>MDVDLGKLFFCGFDDFNEEAREVIQKYRPAGVLIYPGVLSKEYLFLDFMNFLSRNGRFIVSSDHEGGQLEVLKYVPSFPGNLAAGKVDPVFTGRYCEMAGRIMNTLGFNMVFAPVLDLLSEKGSAVVDLRSFGSDPEVVASHGMEACMGYFKGGVIPCIKHFPGHGKTADDSHYLLPTVNASFEELWREDLLPFRRIFQSRVKTAVMTAHVKYPAVDDLPATLSKKLITEVLREKLNFKGLVLSDAMEMKAISENFSVEEAVRFFIEAGGNMILLDNFRDLPVYYESLKKLIEDGSIERGKVERSIKIVDEYLSALENRFNSGLIAEVAERAIECTRMRKELLGREVVLLVPSNKNLSPADTTGDDYDLIPEVAKRFFKVRDVIRYDIEAGPDDVDGELIFDFVVNASKNEQ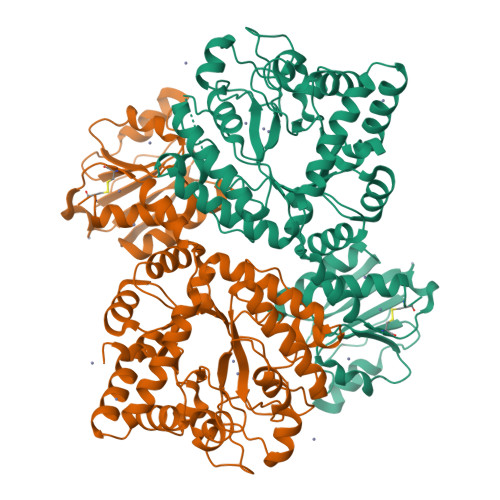VLQAHLSLPSDRTIYFIIRNPFDAKFFPGRSVVITHSTKPISVYKSFQHLLGRCS[4x]> MTTYLEFIQQNEERDGVRFSWNVWPSSRLEATRMVVPVAALFTPLKERPDLPPIQYEPVLCSRTTCRAVLNPLCQVDYRAKLWACNFCYQRNQFPPSYAGISELNQPAELLPQFSSIEYVVLRGPQMPLIFLYVVDTCMEDEDLQALKESMQMSLSLLPPTALVGLITFGRMVQVHELGCEGISKSYVFRGTKDLSAKQLQEMLGLSKVPLTQATRGPQVQQPPPSNRFLQPVQKIDMNLTDLLGELQRDPWPVPQGKRPLRSSGVALSIAVGLLECTFPNTGARIMMFIGGPATQGPGMVVGDELKTPIRSWHDIDKDNAKYVKKGTKHFEALANRAATTGHVIDIYACALDQTGLLEMKCCPNLTGGYMVMGDSFNTSLFKQTFQRVFTKDMHGQFKMGFGGTLEIKTSREIKISGAIGPCVSLNSKGPCVSENEIGTGGTCQWKICGLSPTTTLAIYFEVVNQHNAPIPQGGRGAIQFVTQYQHSSGQRRIRVTTIARNWADAQTQIQNIAASFDQEAAAILMARLAIYRAETEEGPDVLRWLDRQLIRLCQKFGEYHKDDPSSFRFSETFSLYPQFMFHLRRSSFLQVFNNSPDESSYYRHHFMRQDLTQSLIMIQPILYAYSFSGPPEPVLLDSSSILADRILLMDTFFQILIYHGETIA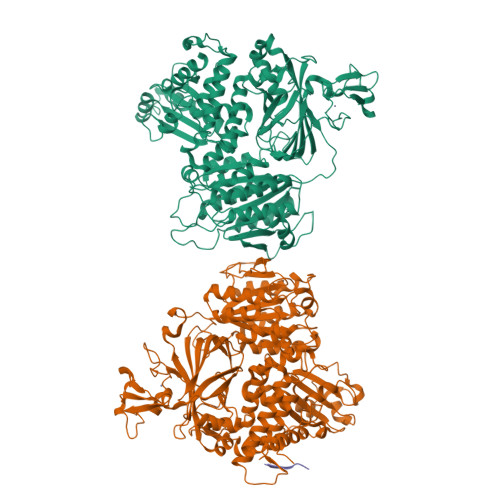QWRKSGYQDMPEYENFRHLLQAPVDDAQEILHSRFPMPRYIDTEHGGSQARFLLSKVNPSQTHNNMYAWGQESGAPILTDDVSLQVFMDHLKKLAVSSA;> AMGSPIQVIENDRASRGGQVYATNTRGQIPPLVTTDCMIQDQGNASPRFIRCTTYCFPCTSDMAKQAQIPLAAVIKPFATIPSNESPLYLVNHGESGPVRCNRCKAYMCPFMQFIEGGRRYQCGFCNCVNDVPPFYFQHLDHIGRRLDHYEKPELSLGSYEYVATLDYCRKSKPPNPPAFIFMIDVSYSNIKNGLVKLICEELKTMLEKIPKEEQEETSAIRVGFITYNKVLHFFNVKSNLAQPQMMVVTDVGEVFVPLLDGFLVNYQESQSVIHNLLDQIPDMFADSNENETVFAPVIQAGMEALKAADCPGKLFIFHSSLPTAEAPGKLKNRDDKKLVNTDKEKILFQPQTNVYDSLAKDCVAHGCSVTLFLFPSQYVDVASLGLVPQLTGGTLYKYNNFQMHLDRQQFLNDLRNDIEKKIGFDAIMRVRTSTGFRATDFFGGILMNNTTDVEMAAIDCDKAVTVEFKHDDKLSEDSGALIQCAVLYTTISGQRRLRIHNLGLNCSSQLADLYKSCETDALINFFAKSAFKAVLHQPLKVIREILVNQTAHMLACYRKNCASPSAASQLILPDSMKVLPVYMNCLLKNCVLLSRPEISTDERAYQRQLVMTMGVADSQLFFYPQLLPIHTLDVKSTMLPAAVRCSESRLSEEGIFLLANGLHMFLWLGVSSPPELIQGIFNVPSFAHINTDMTLLPEVGNPYSQQLRMIMGIIQQKRPYSMKLTIVKQREQPEMVFRQFLVEDKGLYGGSSYVDFLCCVHKEICQLLN;> TTIPMDS> FDCGKPQVEPKKCPGRVVGGCVAHPHSWPWQVSLRTRFGMHFCGGTLISPEWVLTAAHCLEKSPRPSSYKVILGAHQEVNLEPHVQEIEVSRLFLEPTRKDIALLKLSSPAVITDKVIPACLPSPNYVVADRTECFITGWGETQGTFGAGLLKEAQLPVIENKVCNRYEFLNGRVQSTELCAGHLAGGTDSCQGDSGGPLVCFEK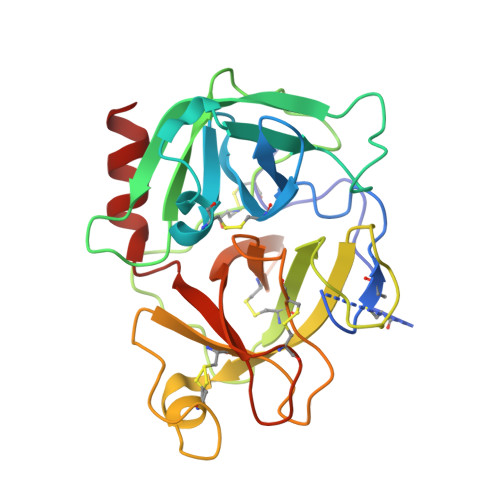DKYILQGVTSWGLGCARPNKPGVYVRVSRFVTWIEGVMRNN(2S,3S,4R,5R)-2-(3,4-diaminophenyl)-5-(hydroxymethyl)pyrrolidine-3,4-diol | C11 H17 N3 O3 | 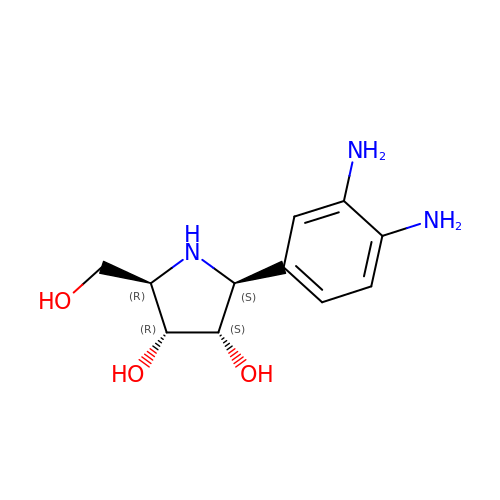YAYMFJWCRXEXGZ-YTWAJWBKSA-N>MAHHHHHHMGFLDGKRILLTGLLSNRSIAYGIAKACKREGAELAFTYVGDRFKDRITEFAAEFGSELVFPCDVADDAQIDALFASLKTHWDSLDGLVHSIGFAPREAIAGDFLDGLTRENFRIAHDISAYSFPALAKAALPMLSDDASLLTLSYLGAERAIPNYNTMGLAKAALEASVRYLAVSLGAKGVRVNAISAGPIKTLAASGIKSFGKILDFVESNSPLKRNVTIEQVGNAGAFLLSDLASGVTAEVMHVDSGFNAVV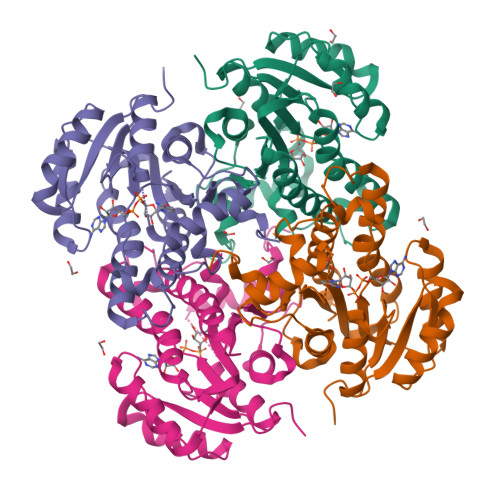GGMAGLEE[4x]>PISPIETVPVKLKPGMDGPKVKQWPLTEEKIKALVEICTEMEKEGKISKIGPENPYNTPVFAIKKKDSTKWRKLVDFRELNKRTQDFWEVQLGIPHPAGLKKKKSVTVLDVGDAYFSVPLDEDFRKYTAFTIPSINNETPGIRYQYNVLPQGWKGSPAIFQSSMTKILEPFKKQNPDIVIYQYMDDLYVGSDLEIGQHRTKIEELRQHLLRWGLTTPDKKHQKEPPFLWMGYELHPDKWTVQPIVLPEKDSWTVNDIQKLVGKLNWASQIYPGIKVRQLSKLLRGTKALTEVIPLTEEAELELAENREILKEPVHGVYYDPSKDLIAEIQKQGQGQWTYQIYQEPFKNLKTGKYARMRGAHTNDVKQLTEAVQKITTESIVIWGKTPKFKLPIQKETWETWWTEYWQATWIPEWEFVNTPPLVKLWYQLEKEPIVGAETFYVDGAANRETKLGKAGYVTNKGRQKVVPLTNTTNQKTELQAIYLALQDSGLEVNIVTDSQYALGIIQAQPDKSESELVNQIIEQLIKKEKVYLAWVPAHKGIGGNEQVDKLVSAG[2x];>MAHHHHHHALEVLFQGPISPIETVPVKLKPGMDGPKVKQWPLTEEKIKALVEICTEMEKEGKISKIGPENPYNTPVFAIKKKD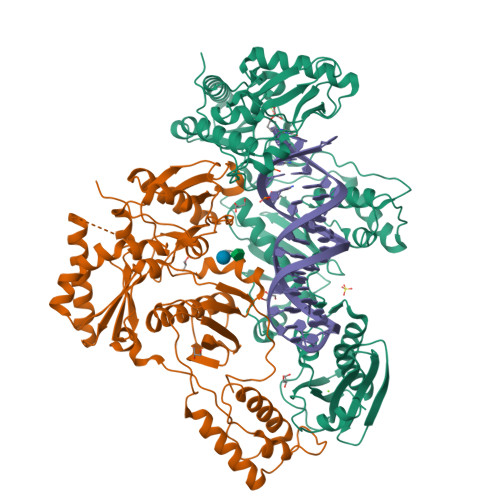STKWRKLVDFRELNKRTQDFWEVQLGIPHPAGLKKKKSVTVLDVGDAYFSVPLDEDFRKYTAFTIPSINNETPGIRYQYNVLPQGWKGSPAIFQSSMTKILEPFKKQNPDIVIYQYMDDLYVGSDLEIGQHRTKIEELRQHLLRWGLTTPDKKHQKEPPFLWMGYELHPDKWTVQPIVLPEKDSWTVNDIQKLVGKLNWASQIYPGIKVRQLSKLLRGTKALTEVIPLTEEAELELAENREILKEPVHGVYYDPSKDLIAEIQKQGQGQWTYQIYQEPFKNLKTGKYARMRGAHTNDVKQLTEAVQKITTESIVIWGKTPKFKLPIQKETWETWWTEYWQATWIPEWEFVNTPPLVKLWYQ[2x]>VMT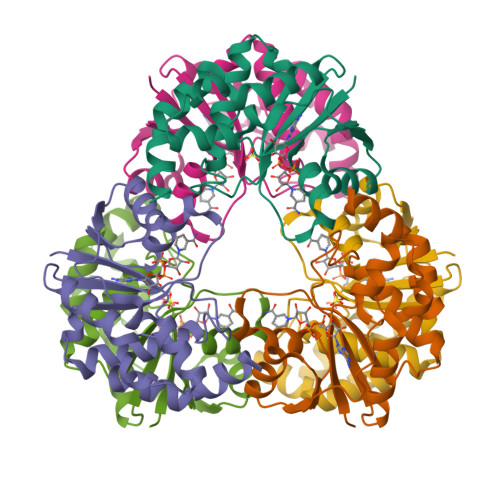MRGLLVGRMQPFHRGALQVIKSILEEVDELIICIGSAQLSHSIRDPFTAGERVMMLTKALSENGIPASRYYIIPVQDIECNALWVGHIKMLTPPFDRVYSGNPLVQRLFSEDGYEVTAPPLFYRDRYSGTEVRRRMLDDGDWRSLLPESVVEVIDEINGVERIKHLAKKEVSELGGIS[3x]>[2x]LVPRGSHMTIDQWLLKNAKEDAIAELKKAGITSDFYFNAINKAKTVEEVNALKNEI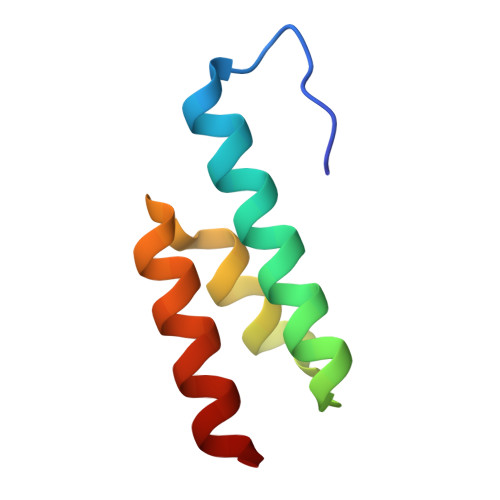LKAHA> MTDNPNKKTFWDKVHLDPTMLLILLALLVYSALVIWSASGQDIGMMERKIGQIAMGLVIMVVMAQIPPRVYEGWAPYLYIICIILLVAVDAFGAISKGAQRWLDLGIVRFQPSEIAKIAVPLMVARFINRDVCPPSLKNTGIALVLIFMPTLLVAAQPDLGTSILVALSGLFVLFLSGLSWRLIGVAVVLVAAFIPILWFFLMHDYQRQRVMMLLDPESDPLGAGYHIIQSKIAIGSGGLRGKGWLHGTQSQLEFLPERHTDFIFAVLAEELGLVGILILLALYILLIMRGLWIAARAQTTFGRVMAGGLMLILFVYVFVNIGMVSGILPVVGVPLPLVSYGGSALIVLMAGFGIVMSIHTHRKMLSKSV;> MKLQNSFRDYTAESALFVRRALVAFLGILLLTGVLIANLYNLQIVRFTDYQTRSNENRIKLVPIAPSRGIIYDRNGIPLALNRTIYQIEMMPEKVDNVQQTLDALRSVVDLTDDDIAAFRKERARSHRFTSIPVKTNLTEVQVARFAVNQYRFPGVEVKGYKRRYYPYGSALTHVIGYVSKINDKDVERLNNDGKLANYAATHDIGKLGIERYYEDVLHGQTGYEEVEVNNRGRVIRQLKEVPPQAGHDIYLTLDLKLQQYIETLLAGSRAAVVVTDPRTGGVLALVSTPSYDPNLFVDGISSKDYSALLNDPNTPLVNRATQGVYPPASTVKPYVAVSALSAGVITRNTTLFDPGWWQLPGSEKRYRDWKKWGHGRLNVTRSLEESADTFFYQVAYDMGIDRLSEWMGKFGYGHYTGIDLAEERSGNMPTREWKQKRFKKPWYQGDTIPVGIGQGYWTATPIQMSKALMILINDGIVKVPHLLMSTAEDGKQVPWVQPHEPPVGDIHSGYWELAKDGMYGVANRPNGTAHKYFASAPYKIAAKSGTAQVFGLKANETYNAHKIAERLRDHKLMTAFAPYNNPQVAVAMILENGGAGPAVGTLMRQILDHIMLGDNNTDLPAENPAVAAAEDH

PG assembly requires a glycosyltransferase (GT) to generate a glycan polymer using a Lipid II substrate, which is then crosslinked to the existing PG via a transpeptidase (TP) reaction. In E. coli, the GT RodA from the Shape, Elongation, Division, and Sporulation (SEDS) family, and PBP2, the monofunctional TP class B Penicillin Binding Protein, mediate these respective enzymatic tasks. In the periplasm, PG biosynthesis begins with a Lipid II-specific glycosyltransferase (GT) which forms a glycan strand polymer by linking the disaccharides of two Lipid II molecules, one termed the donor and the other the acceptor, and thereby releasing Und-PP from the donor site.

Here, we used single-particle cryo-electron microscopy (cryo-EM) to determine the structure of the E. coli RodA-PBP2 complex, expressed as a functional fusion and reconstituted in lipid-filled nanodiscs, to 3.0 Å resolution. The structure shows ten RodA TM helices, with intracellular N- and C-termini. TM helices 1-6 and TM helices 8–10 form a tight helical bundle, with TM helix 7 extending away from it, stabilized by three periplasmic juxtamembrane helices (PH1, PH2 and PH3). Additionally, the PBP2 single TM helix, is ordered and packs against RodA TM helices 8 and 9. Analysis of the RodA portion of the structure for putative substrate-binding sites reveals two major cavities (termed cavity A and B). Cavity A is located between TM helices 6, 7 and 9, and is framed on one side by PH1 and on the other by TM helices 5 and 6 and the periplasmic loop (PL3) connecting the two. Cavity B is located on the opposite side of RodA relative to cavity A, between TM helices 2, 3, 4 and 10 and is also exposed to the membrane. The region connecting the two cavities has some of the highest degree of conservation in the entire structure. Given their orientation in respect to the TP site of PBP2, we suggest that cavities A and B are the donor and acceptor sites for the two substrates, respectively. In our cryo-EM map, within the putative donor site there is a lipid-like density, which we tentatively assigned to Und-PP, a product of the GT reaction. Within the highly conserved region between the two cavities and centrally located in periplasmic loop 4 (PL4) is Asp262, previously identified as a catalytic residue15,17,29.>[4x]PNYKLTYFNMRGRAEIIRYIFAYLDIQY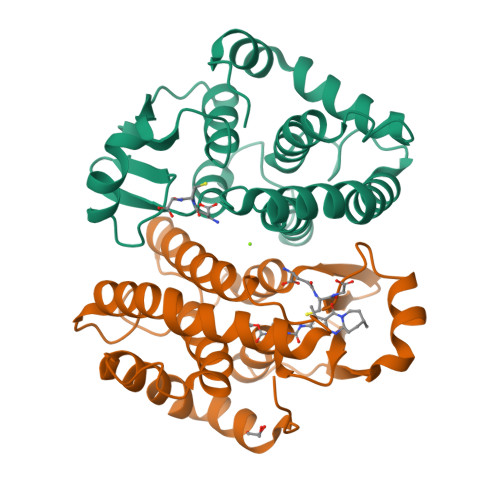EDHRIEQADWPEIKSTLPFGKIPILEVDGLTLHQSLAIARYLTKNTDLAGNTEMEQCHVDAIVDTLDDFMSCFPWAEKKQDVKEQMFNELLTYNAPHLMQDLDTYLGGREWLIGNSVTWADFYWEICSTTLLVFKPDLLDNHPRLVTLRKKVQAIPAVANWIKRRPQTKL>[2x]GPGSMTVVEAKSRIAVVGGGGSGSVAAWLLARRHDVTLFEADEYLGGHAYSHPVETDQGTLHVDMGVEHFNEKLSPNLFRLLTDFGIGTYVAPSSVHVDFPGEQQSWNNLDFLGELREELHEEFDRFHQEMNQLP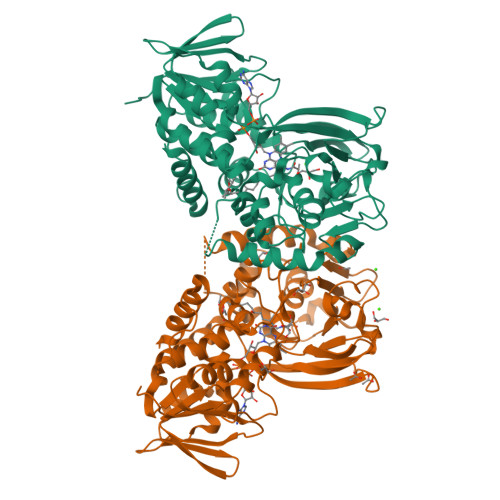TSGDDSYKQMSIGEYLDKHGYSKSFKYKAMNPILSIYSGCHAPSLDYNLMYVALSFSMNLLSFFSAGYWRKAQGGIHSYLARIESDLGERVRLNTPVEAVVPTQSGVTVLAGGQEHHFDQVVFATHADVTLRLLRTSDQQYRDLLGDFAYVPVESVLHQDESWLSPAGGGAYCQFRMPEGFELARAEEQMGSLTQNCNVLHPYRKVSSPILITFDPQEDVDPERVIVRREWKLPQLRPVDVRRKKRLHEIQGLNGLWFCGTDTSVTGHEGAIVSGMVIADRLGVPHPFPDDAPAAAQFRGIKEFMGV>[2x]VEDVCTAKPRDIPVNPMCIYRSSEKKATEGQGSEQKIPGATNRRVWELSKANSHFATAFYQHLADSKNNNDNIFLSPLSISTAFAMTKLGACNNTLTQLMEVFKFDTISEKTSDQIHFFFAKLNCRLYRKANKSSELVSANRLFGDKSITFNETYQDISEVVYGAKLQPLDFKGNAEQSRLTINQWISNKTEGRITDVIPPQAINEFTVLVLVNTIY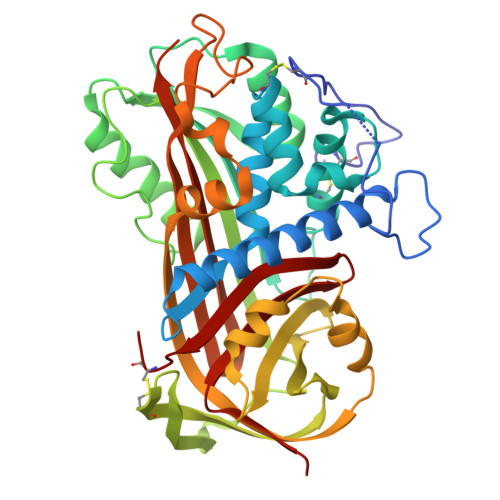FKGLWKSKFSPENTRKELFYKADGESCSVLMMYQESKFRYRRVAESTQVLELPFKGDDITMVLILPKLEKTLAKVEQELTPDMLQEWLDELTETLLVVHMPRFRIEDSFSVKEQLQDMGLEDLFSPEKSRLPGIVAEGRSDLYVSDAFHKAFLEVNEEGSEAAASTVISIAGRSLNSDRVTFKANRPFLVLIREVALNTIIFMGRVANPCVD(2E)-2-{[(Z)-{3-HYDROXY-2-METHYL-5-[(PHOSPHONOOXY)METHYL]PYRIDIN-4(1H)-YLIDENE}METHYL]IMINO}PROPANOIC 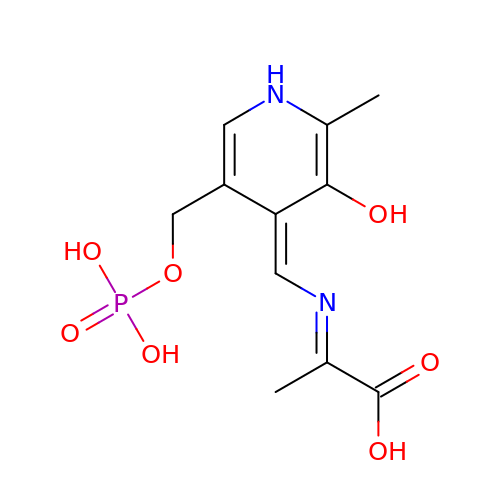ACID | C11 H15 N2 O7 P | ADVVJYVQWSKPQC-ZAQQZXBOSA-N> HNHNHNHNHNHNGGENLYFQGASLTEIEHLVQSVCKSY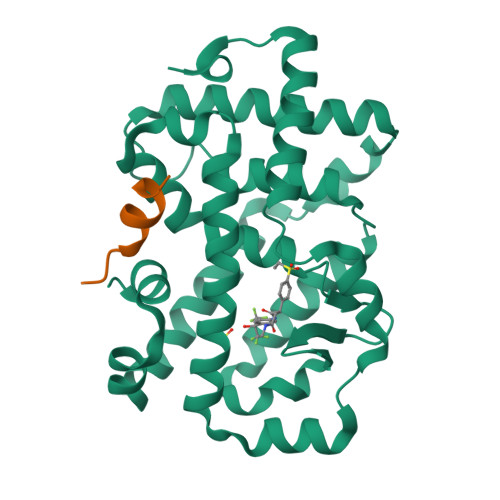RETCQLRLEDLLRQRSNIFSREEVTGYQRKSMWEMWERCAHHLTEAIQYVVEFAKRLSGFMELCQNDQIVLLKAGAMEVVLVRMCRAYNADNRTVFFEGKYGGMELFRALGCSELISSIFDFSHSLSALHFSEDEIALYTALVLINAHRPGLQEKRKVEQLQYNLELAFHHHLCKTHRQSILAKLPPKGKLRSLCSQHVERLQIFQHLHPIVVQAAFPPLYKELFSGG;> GGGKEKHKILHRLLQDSS6-{[(3S,4S)-4-{[(4E)-5-(3-fluorophenyl)pent-4-en-1-yl]oxy}pyrrolidin-3-yl]methyl}-4-methylpyridin-2-amine 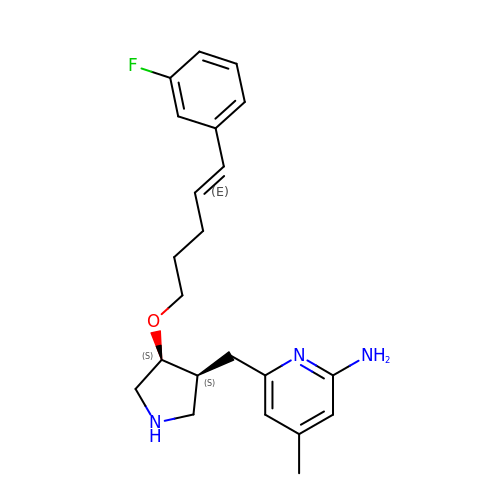| C22 H28 F N3 O | GPCIKCOFIVHWEN-KAMCARKFSA-N2-(decylamino)ethane-1-thiol | C12 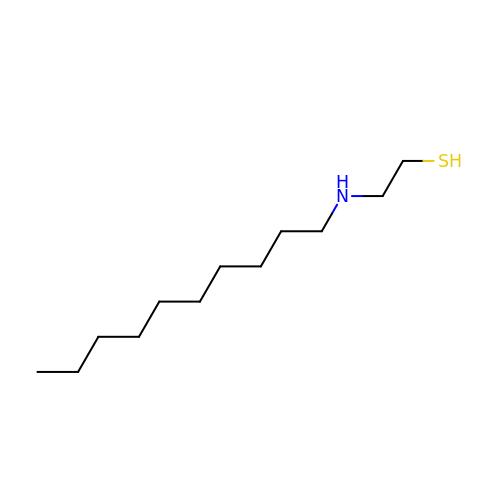H27 N S | WOWHRXFAFVDNAP-UHFFFAOYSA-N> MKFSVIVPTYNSEKYITELLNSLAKQDFPKTEFEVVVVDDCSTDQTLQIVEKYRNKLNLKVSQLETNSGGPGKPRNVALKQAEGEFVLFVDSDDYINKETLKDAAAFIDEHHSDVLLIKMKGVNGRGVPQSMFKETAPEVTLLNSRIIYTLSPTKIYRTALLKDNDIYFPEELKSAEDQLFTMKAYLNANRISVLSDKAYYY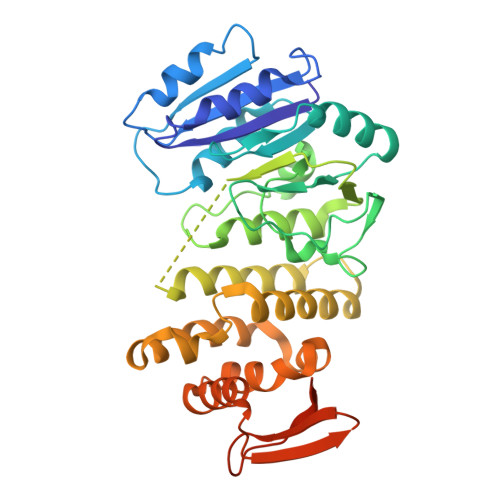ATKREGEHMSSAYVSPEDFYEVMRLIAVEILNADLEEAHKDQILAEFLNRHFSFSRTNGFSLKVKLEEQPQWINALGDFIQAVPERVDALVMSKLRPLLHYARAKDIDNYRTVEESYRQGQYYRFDIVDGKLNIQFNEGEPYFEGIDKLVPRGSAAAALEHHHHHH>[4x]AGEARLEEAVNRWVLKFYFHEALRAFRGSRYGDFRQIRDIMQALLV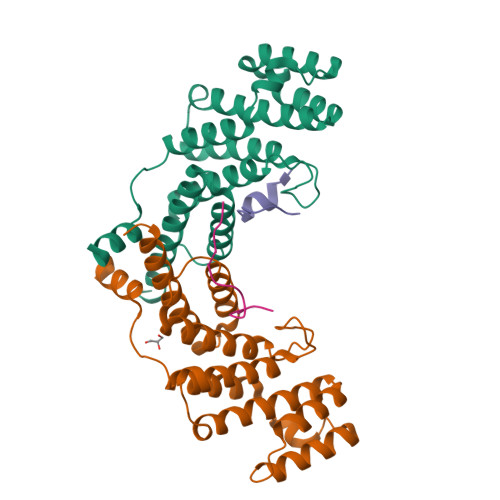RPLGKEHTVSRLLRVMQCLSRIEEGENLDCSFDMEAELTPLESAINVLEMIKTEFTLTEAVVESSRKLVKEAAVIICIKNKEFEKASKILKKHMSKDPTTQKLRNDLLNIIREKNLAHPVIQNFSYETFQQKMLRFLESHLDDAEPYLLTMAKKALK;>ENRERLELEAYRLGPASA[4x]> MAPEYDYLFKLLLIGDSGVGKSCLLLRFADDTYTESYISTIGVDFKIRTIELDGKTIKLQIWDTAGQERFRTITSSYYXGAHGIIVVYDVTDQESYA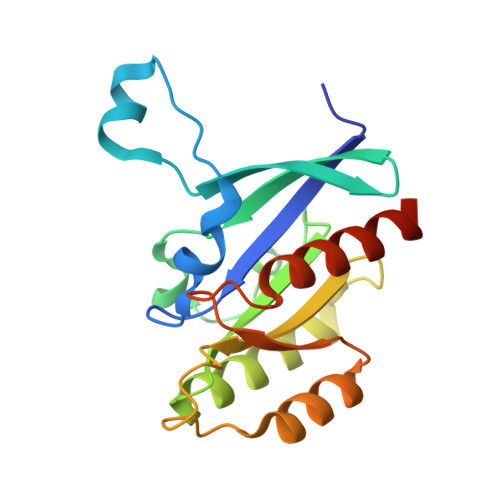NVKQWLQEIDRYASENVNKLLVGNKSDLTTKKVVDNTTAKEFADSLGIPFLETSAKNATNVEQAFMTMAAEIKKRMGHHHHHH> SLDDDVLIVYELTPTAEQKALATKLKLPPTFFCYKNRPDYVSEEEED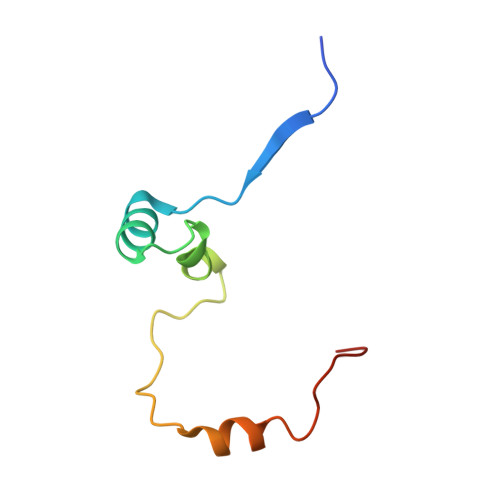DEDFETAVKKLNGKLYLDGSEK>GSACAEFSFHVPSLEELAGVMQKGLKDNFADVQVSVVDCPDLTKEPFTFPVKGICGKTRIAEVGGVPYLLPLVNQKKVYDLNKIAKEIKLPGAFILGAGAGPFQTLGFNSEFMPVIQTESEHKPPVNGSYFAHVNPADGGCLLEKYSE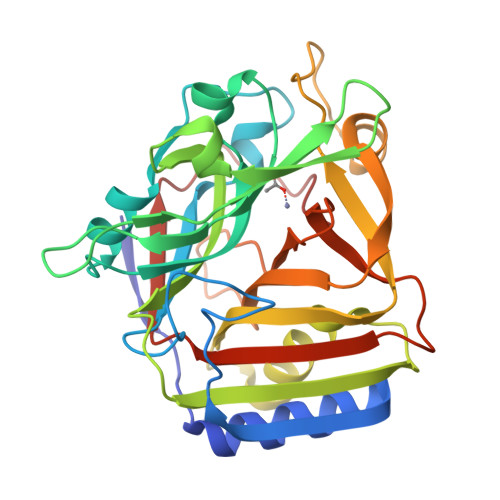KCHDFQCALLANLFASEGQPGKVIEVKAKRRTGPLNFVTCMRETLEKHYGNKPIGMGGTFIIQKGKVKSHIMPAEFSSCPLNSDEEVNKWLHFYEMKAPLVCLPVFVSRDPGFDLRLEHTHFFSRHGEGGHYHYDTTPDIVEYLGYFLPAEFLYRIDQPKETHSIGRD[2x]The endo-chitinase Chit33 from T. harzianum is included in the GH18 family. Chit33 belongs to class III (plant-type) enzymes characterized by the presence of shallow catalytic tunnels and open substrate-binding grooves. Chit33 is folded into a (β/α)8 barrel domain, similarly to family 18 chitinases. The DxDxEx conserved catalytic motif is located at the end of strand β4 of the barrel, with Glu167 being the catalytic acid protonating the glycosidic bond and Asp165 playing a key role in assisting the acetamido group in its nucleophilic attack and stabilizing the developing positive charge on the oxazolinium ion.

To further investigate the substrate binding mode and to provide a platform for rational mutant design, we determined the crystal structure of the inactive double-mutant D165A/E167A with the substrate NAG4. The inactivated double-mutant D165A/E167A was also crystallized and used for soaking experiments with a series of chito-oligosaccharides (COS); however, only NAG4 was captured at the Chit33 active site, although a cocrystallization technique was also attempted with NAG3, NAG5 and NAG6. A clear electron density is observed for the tetrasaccharide, spanning subsites −2, −1, +1 and +2. All the subsites are highly defined though a large number of polar interactions that tightly fix the sugar. At subsite −1, the boat sugar conformation postulated for the bound substrate in a state previous to oxazinium intermediate formation was crystallographically trapped. Previous structural and kinetic studies on hevamine proposed the combined action of Asp125 and Tyr183 (Asp165 and Tyr224 in Chit33) in positioning the carbonyl oxygen of the N-acetyl group at position −1 near to the C1 atom, which would stabilize the positively charged transient intermediate during substrate-assisted nucleophilic attack. In our study, although we succeeded in trapping the distorted boat conformation of the substrate at subsite −1, these hydrogen-bonding interactions are lost in our double D165A/E167A mutant, which results in a flip of the N-acetyl group that locates its oxygen carbonyl away from the C1 atom. Structural comparison of the wild type and the complex with NAG4 Chit33 does not show significant differences, apart from a visible reorganization of the Asp117 and Arg274 side chains that approach the substrate, enabling direct polar links. In summary, the major structural trait of the Chit33 binding site is the presence of the non-conserved residues Asp117 and Arg274, which act as a clamp that may fix the bent conformation of the substrate that occupies the full catalytic groove, conversely to that reported in hevamine. Nevertheless, it is remarkable that we failed to trap the Chit33-NAG6 complex—an issue that can be explained by looking to the crystal packing, which shows that the non-reducing positions of the active site are blocked by the small loop following α8 (Ala187-Lys192) from a symmetry-related molecule.

> AGWNVNSKQNIAVYWGQNSANSQSTQQRLSFYCNDANINVIDIAFLNGITPPMTNFANAGDRCTPFSDNPWLLQCPEIEADIKTCQANGKTILLSLGGDSYTQGGWSSTGAAQSAADQVWAMFGPVQSGSSVHRPFGSAVVDGFDFAFAATTNNLAAFGAQLKSRTNAAGGKKYYFSAAPQCFFPDAAVGALINAVPMDWIQIQFYNNPCGVSGFTPGTSTQNNYNYQTWENWAKTSPNPNVKLLVGIPAGPGAGRGYVSGSQLTSVFQYSKGFSTFAGAMMWDMSQLYQNTGFETQVVNALR>AANAPGGSNVVNETPAQTVEVRAA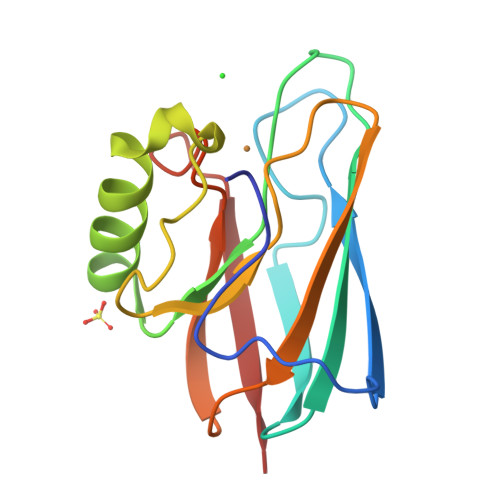PDALAFAQTSLSLPANTVVRLDFVNQNNLGVQHNWVLVNGGDDVAAAVNTAAQNNADALFVPPPDTPNALAWTAMLNAGESGSVTFRTPAPGTYLYICTFPGHYLAGMKGTLTVTP[4x]> MKTEWPELVGK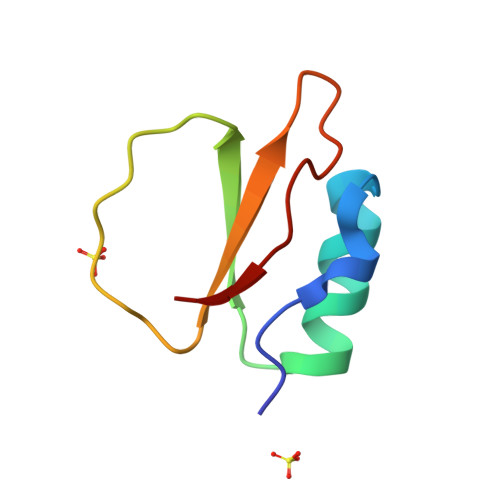SVEEAKKVILQDKPEAQIIVLPVGTIVTMEYRIDRVRIFVDKLDNIAQVPRVG> GLVPRGSHMTGRMLTLDGNPAANWLNNARTKWSASRADVVLSYQQNNGGWPKNLDYNSVGNGGGGNESGTIDNGATITEMVFLAEVYKSGGNTKYRDAVRKAANFLVNSQYSTGALPQFYPLKGGYSDHATFNDNGMAYALTVLDFAANKRAPFDTDVFSDNDRTRFKTAVTKGTDYILKAQWKQNGVLTVWCAQHGALDYQPKKARAYELESLSGSESVGVLAFLMTQPQTAEIEQAVRAGVAWFNSPRTYLEGYTYDSSLAATNPIVPRAGSKMWYRFYDLNTNRGFFSDRDGSKFYDITQMSLERR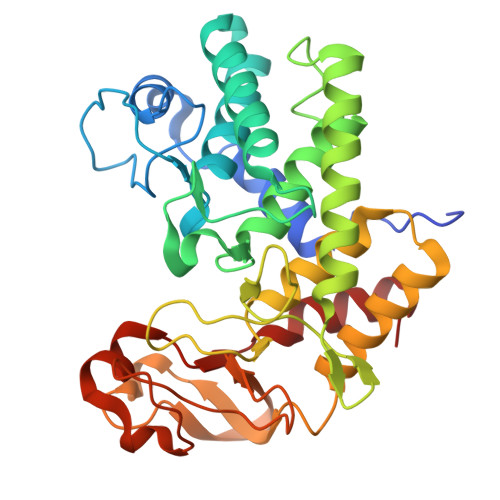TGYSWGGNYGTSIINFAQKVGYL>[4x]MAHHHHHHMLNDPEARMVANCPVLVTGGARRIGKAIVEDLASHGFPVAIHCNRSLDEGEAIANRINDSGGNACVVQADLEGDVRGLVKQASDRIGPIRLLVNNASLFQEDKVGALDMALWDRHFAVHLKTPVILAEDMRKALPEDQDGLVVNIIDQRVWKLNPQFFSYTLSKSALWNATRTLAQALAPRIRVNAIAPGPTLPSERQRPEDFERQVSKLPLQRAPELPEFGRTVRYFWENRSITGQMIALDGGQHLAWETPDIAGITE

Dihydrofolate reductase reduces dihydrofolic acid to tetrahydrofolic acid using reduced nicotinamide adenine dinucleotide phosphate (NADPH) as the electron donor. While this reaction is catalyzed by the enzyme dihydrofolate reductase (DHFR) in mammals and other organisms, some bacteria have an alternative pathway for reduced folate biosynthesis using FolM alternative di­hydrofolate reductase 1. Here, we present the crystal structures of FolM alternative dihydro­folate reductase 1 from two Brucella species, B. suis (BsFolM) and B. canis (BcFolM). BsFolM and BcFolM are 95% identical in sequence.

The interface interactions are mostly hydrogen bonds and other nonbonded contacts. The tetramers are similar and superpose with an r.m.s.d. of ∼0.5 Å. Each monomer has the extended double-Rossmann fold of NADPH-dependent SDRs with a central seven-stranded parallel β-sheet sandwiched between two pairs of three α-helices. Both the BsFolM and BcFolM structures were co-crystallized with a cofactor (NADPH). The BsFolM and BcFolM structures are in the closed conformation with ordered substrate-binding loops, as observed in protozoan pteridine reductases. Apart from this loop region, the cofactor-binding cavity is very similar in these enzymes. Furthermore, the residues involved in NADPH binding are well conserved. While the substrates of BsFolM and BcFolM are unknown, their substrate-binding cavities are large enough to accommodate the inhibitors identified by rational therapeutics discovery for human African trypanosomiasis and Chagas disease.> ELICIVQRVNESFSLHSGFGGNVYSMKTEPMTGFTNVTKGASVINQKDWIGFGDSRTDLTNDQFPASSDVPLAVAKKFRSLSGASLMLSAFGPPGKVDYLYQGCGKEKVFYEGVNWSPEAGIDCFGSNWTQTKKDFYSRIYEAARSSTCMTLVNSLDTKISSTTATAGTASS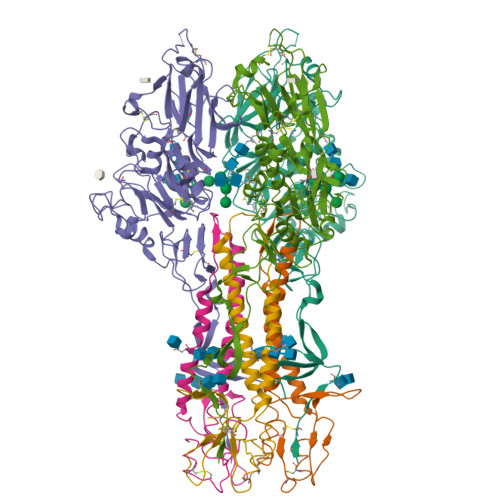CSSSWMKSPLWYAESSVNPGAKPQVCGTEQSATFTLPTSFGIYKCNKHVVQLCYFVYENKAKFNTFGCGDYYQNYYDGNGNLIGGMDNRVAAYRGIANAGVKIECPSKILNPGTYSIKSTPRFLLVPKRSYCFDTDGGYPIQVVQSEWSASRRSDNATEEACLQTEGCIFIKKTTPYVGEADDNHGDIEMRQLLSGLGNNDTVCVSQSGYTKGETPFVKDYLSPPKYGRCQLKTDSGRIPTLPSGLIIPQAGTDS;> IFGIDDLIFGLLFVGFVAGGVAGGYFWGRSNGGGGGASVSSTQAGFDKIGKDIQQLRNDTNAAIEGFNGRIAHDEQAIKNLAKEIEDARAEALVGELGIIRSLIVANISMNLKESLYELANQITKRGGGIAQEAGPGCWYVDSENCDASCKEYIFNFNGSATVPTL> MELWMVRHGETLWNREGRLLGWTDLPLTAEGEAQARRLKGALPSLPAFSSDLLRARRTAELAGFSPRLYPELREIHFGALEGALWETL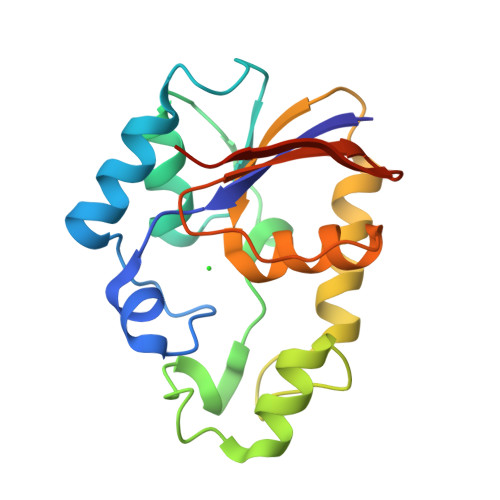DPRYKEALLRFQGFHPPGGESLSAFQERVFRFLEGLKAPAVLFTHGGVVRAVLRALGEDGLVPPGSAVAVDWPRRVLVRLALDGEEATG5alpha-dihydronandrolone 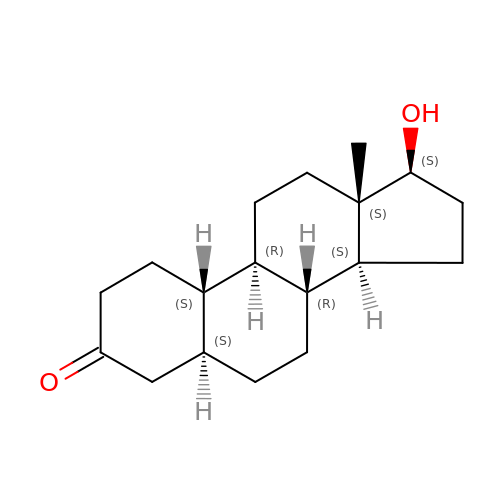| C18 H28 O2 | RHVBIEJVJWNXBU-PNOKGRBDSA-N> MSETRMAQNMDTTDEQYLRLIELLSNYDSTLEQLQKGFQDGYIQLSRSNYYNKDSLRGNYGEDYWDETYIGQLMATVEEKNSKVVVEIVKRKAQDKQEKKEEEDNKLTQRKKGTKPEKQKTQSHKLKQDYDPILMFGGVLSVPSSLRQSQTSFKGCIPLIAQLINYKNEILTLVETLSEQE;> MAEKRTLIAVIADEDTTTGLLLAGIGQITPETQEKNFFVYQEGKTTKEEITDKFNHFTEERDDIAILLINQHIAENIRARVDSFTNAFPAILEIPSKDHPYDPEKDSVLKRVRKLFGE;> MAEKEEAIFRSAEMALVQFYIPQEISRDSAYTLGQLGLVQFRDLNSKVRAFQRTFVNEIRRLDNVERQYRYFYSLLKKHDIKLYEGDTDKYLDGSGELYVPPSGSVIDDYVRNASYLEERLIQMEDATDQIEVQKNDLEQYRFILQSGDEFFLKGDNTDSTSYMDEDMIDANGENIAAAIGASVNYVTGVIARDKVATLEQILWRVLRGNLFFKTVEIEQPVYDVKTREYKHKNAFIVFSHGDLIIKRIRKIAESLDANLYDVDSSNEGRSQQLAKVNKNLSDLYTVLKTTSTTLESELYAIAKELDSWFQDVTREKAIFEILNKSNYDTNRKILIAEGWIPRDELATLQARLGEMIARLGIDVPSIIQVLDTNHTPPTFHRTNKFTAGFQSICDCYGIAQYREINAGLPTIVTFPFMFAIMFGDMGHGFLMTLAALSLVLNEKKINKMKRGEIFDMAFTGRYIILLMGVFSMYTGFLYNDIFSKTMTIFKSGWKWPDHWKKGESITATSVGTYPIGLDWAWHGTENALLFSNSYKMKLSILMGFIHMTYSYFFSLANHLYFNSMIDIIGNFIPGLLFMQGIFGYLSVCIVYKWAVDWVKDGKPAPGLLNMLINMFLSPGTIDDELYPHQAKVQVFLLLMALVCIPWLLLVKPLHFKFTHKKKSHEPLPSTEADASSEDLEAQQLISAMDADDAEEEEVGSGSHGEDFGDIMIHQVIHTIEFCLNCVSHTASYLRLWALSLAHAQLSSVLWTMTIQIAFGFRGFVGVFMTVALFAMWFALTCAVLVLMEGTSAMLHSLRLHWVESMSKFFVGEGLPYEPFAFEYKDMEVAVASASSSASS;> MVFGQLYALFIFTLSCCISKTVQADSSKESSSFISFDKESNWDTISTISSTADVISSVDSAIAVFEFDNFSLLDNLMIDEEYPFFNRFFANDVSLTVHDDSPLNISQSLSPIMEQFTVDELPESASDLLYEYSLDDKSIVLFKFTSDAYDLKKLDEFIDSCLSFLEDKSGDNLTVVINSLGWAFEDEDGDDEYATEETLSHHDNNKGKEGDDDILSSIWTEGLLMCLIVSALLLFILIVALSWISNLDITYGALEKSTNPIKKNN;> MNKESKDDDMSLGKFSFSHFLYYLVLIVVIVYGLYKLFTGHGSDINFGKFLLRTSPYMWANLGIALCVGLSVVGAAWGIFITGSSMIGAGVRAPRITTKNLISIIFCEVVAIYGLIIAIVFSSKLTVATAENMYSKSNLYTGYSLFWAGITVGASNLICGIAVGITGATAAISDAADSALFVKILVIEIFGSILGLLGLIVGLLMAGKASEFQ;> MEGVYFNIDNGFIEGVVRGYRNGLLSNNQYINLTQCDTLEDLKLQLSSTDYGNFLSSVSSESLTTSLIQEYASSKLYHEFNYIRDQSSGSTRKFMDYITYGYMIDNVALMITGTIHDRDKGEILQRCHPLGWFDTLPTLSVATDLESLYETVLVDTPLAPYFKNCFDTAEELDDMNIEIIRNKLYKAYLEDFYNFVTEEIPEPAKECMQTLLGFEADRRSINIALNSLQSSDIDPDLKSDLLPNIGKLYPLATFHLAQAQDFEGVRAALANVYEYRGFLETGNLEDHFYQLEMELCRDAFTQQFAISTVWAWMKSKEQEVRNITWIAECIAQNQRERINNYISVY;> MSSFYTVVGVF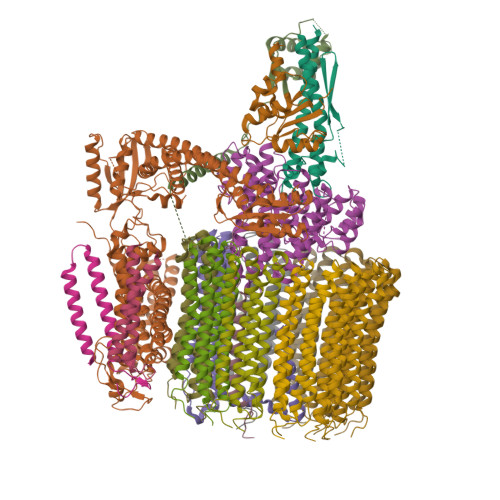IVVSAMSVLFWIMAPKNNQAVWRSTVILTLAMMFLMWAITFLCQLHPLVAPRRSDLRPEFAE;> MRPVVSTGKAWCCTVLSAFGVVILSVIAHLFNTNHESFVGSINDPEDGPAVAHTVYLAALVYLVFFVFCGFQVYLARRKPSIELR;>[8x]MTELCPVYAPFFGAIGCASAIIFTSLGAAYGTAKSGVGICATCVLRPDLLFKNIVPVIMAGIIAIYGLVVSVLVCYSLGQKQALYTGFIQLGAGLSVGLSGLAAGFAIGIVGDAGVRGSSQQPRLFVGMILILIFAEVLGLYGLIVALLLNSRATQDVVC;> MSTQLASNIYAPLYAPFFGFAGCAAAMVLSCLGAAIGTAKSGIGIAGIGTFKPELIMKSLIPVVMSGILAIYGLVVAVLIAGNLSPTEDYTLFNGFMHLSCGLCVGFACLSSGYAIGMVGDVGVRKYMHQPRLFVGIVLILIFSEVLGLYGMIVALILNTRGSE The sterile alpha-motif (SAM) and histidine-aspartate (HD) domain-containing protein 1 (SAMHD1) is a dNTP phosphohydrolase that restricts viral replication by limiting the cellular dNTP pool. The active tetramer form of SAMHD1 is induced by cellular nucleotides, which bind two allosteric sites of each subunit. The SAM domain is not required for dNTP hydrolysis and viral restriction by hSAMHD1, but is essential for these activities of mSAMHD1. To better understand the regulatory role of the SAM domain, we crystallized full-length mSAMHD1 in three different states (0, 1, and 2 allosteric nucleotides bound).

In addition to the 2-Allo structure, we also captured crystal structures of full-length mSAMHD1 in two more activation intermediate states: no allosteric nucleotides bound (No-Allo) and one allosteric nucleotide bound to Allo-site 1 only (1-Allo). The No-Allo crystal was obtained without the addition of nucleotides in the crystallization mixture and diffracted to 3.5 Å resolution. The 1-Allo crystal was crystallized with dGTP-α-S in the crystallization mixture and diffracted to 3.4 Å resolution. The No-Allo and 1-Allo mSAMHD1 structures also crystallized as tetramers in different space groups (C2 and P21212) with 4 or 2 copies of mSAMHD1 in the asymmetric unit, respectively. Our No-Allo and 1-Allo structures show that these inactive tetramer intermediates are composed of two relatively rigid dimers with loose tetramer interfaces. Although mSAMHD1 is capable of forming tetramers without nucleotides bound to Allo-site 2, these states are inactive and likely represent activation intermediates of the enzyme. In the absence of nucleotides, mSAMHD1 exists in an equilibrium between stable dimers and inactive tetramers. Starting from the most open No-Allo state, dimer A′ swings progressively toward dimer A via the 1-Allo-state to close the tetramer interface in the 2-Allo state.

>MGSSHHHHHHSSGLMDSLLGCGVSAAAREPVPRYLTSQPRVSEVAMQSAPLEQPAKRPRCDGSPRTPPSTPPATANLSADDDFQNTDLRTWEPEDVCSFLENRGFREKKVLDIFRDNKIAGSFLPFLDEDRLEDLGVSSLEERKKMIECIQQLSQSRIDLMKVFNDPIHGHIEFHPLLIRIIDTPQFQRLRYIKQLGGGYYVFPGASHNRFEHSLGVGYLAGCLVRALAEKQPELQISERDILCVQIAGLCHDLGHGPFSHMFDGRFIPRARPEKKWKHEQGSIEMFEHLVNSNELKLVMKNYGLVPEEDITFIKEQIMGPPITPVKDSLWPYKGRPATKSFLYEIVSNKRNGIDVDKWDYFARDCHHLGIQNNFDYKRFIKFARICEVEYKVKEDKTYIRKVKHICSREKEVGNLYDMFHTRNCLHRRAYQHKISNLIDIMITDAFLKADPYVEITGTAGKKFRISTAIDDMEAFTKLTDNIFLEVLHSTDPQLSEAQSILRNIECRNLYKYLGETQPKREKIRKEEYERLPQEVAKAKPEKAPDVELKAEDFIVDVINVDYGMEDKNPIDRVHFYCKSNSKQAVRINKEQVSQLLPEKFAEQLIRVYCKKKDGKSLDAAGKHFVQWCALRDFTKPQDGDIIAPLITPLKWNNKTSSCLQEVSKVKTCLKF[4x]>[2x]MALLERILARDNLITALKRVEANQGAPGIDGVSTDQLRDYIRAHWSTIHAQLLAGTYRPAPVRRVEIPKPGGGTRQLGIPTVVDRLIQQAILQELTPIFDPDFSSSSFGFRPGRNAHDAVR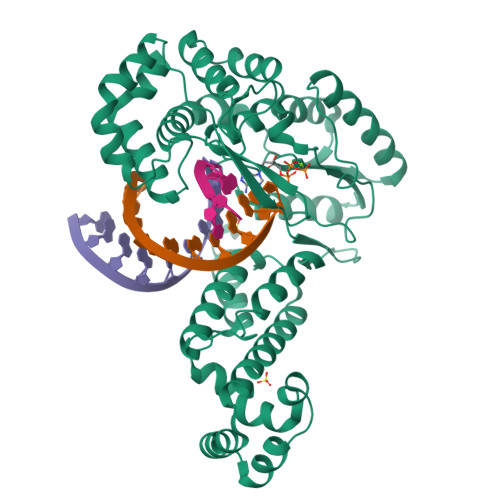QAQGYIQEGYRYVVDMDLEKFFDRVNHDILMSRVARKVKDKRVLKLIRAYLQAGVMIEGVKVQTEEGTPQGGPLSPLLANILLDDLDKELEKRGLKFCRYADDCNIYVKSLRAGQRVKQSIQRFLEKTLKLKVNEEKSAVDRPWKRAFLGFSFTPERKARIRLAPRSIQRLKQRIRQLTNPNWSISMPERIHRVNQYVMGWIGYFRLVETPSVLQTIEGWIRRRLRLCQWLQWKRVRTRIRELRALGLKETAVMEIANTRKGAWRTTKTPQLHQALGKTYWTAQGLKSLTQRYFELRQGHHHHHHHH> NTFEDFYLKRELLMGIFEAGFEKPSPIQEEAIPVAITGRDILARAKNGTGKTAAFVIPTLEKVKPKLNKIQALIMVPTRELALQTSQVVRTLGKHCGISCMVTTGGTNLRDDILRLNETVHILVGTPGRVLDLASRKVADLSDCSLFIMDEADKMLSRDFKTIIEQILSFLPPTHQSLLFSATFPLTVDEFMDKHLHKPYEINLMEELTLKGITQYYAFVEERQKLHCLNTLFSKLQINQAIIFCNSTNRVELLAKKITDLGYSCYYSHARMKQQERNKVFHEFRQGKVRTLVCSDLLTRGIDI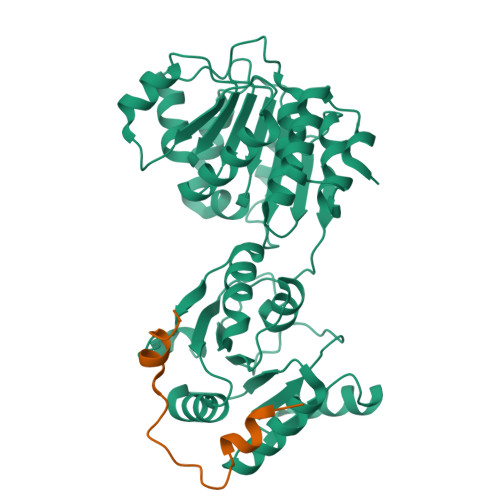QAVNVVINFDFPKTAETYLHRIGRSGRFGHLGLAINLINWNDRFNLYKIEQELGTEIAAIPATIDKSLYVAEN;> RSMQQNDYNQNRGEHIDWQDDDVSKIKQQEDFDFQRNLGMFNK> SCAIDQDFLDAAGILENEAIDIWNVTNGKRFSVYAIAAERGSRIISVNGAAAHCASVGDIVIIASFVTMPDEEARTWRPN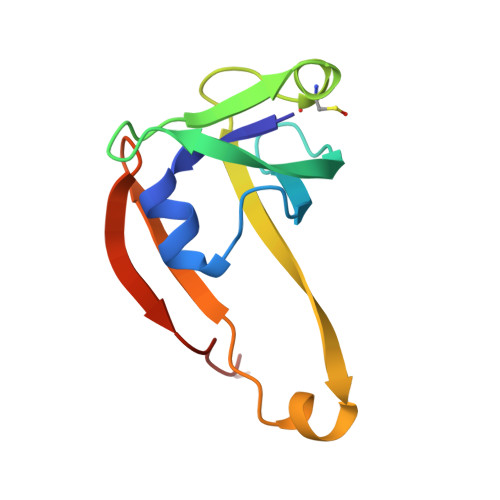VAYFEGDNEMKRTAKAIPVQVA> GETGQLIKDTIKNTVENTVESTHSISTEATPALQAAETGATSNASDESMIETRNVVNTHGVAETSLEGFYGRAGLVAMFTTEGGIRSWYINFGKYVQLRAKLELLTYARFDVEFTIVAQVVDEQAKVKDFNVDYQVMYVPPGASAPDGQ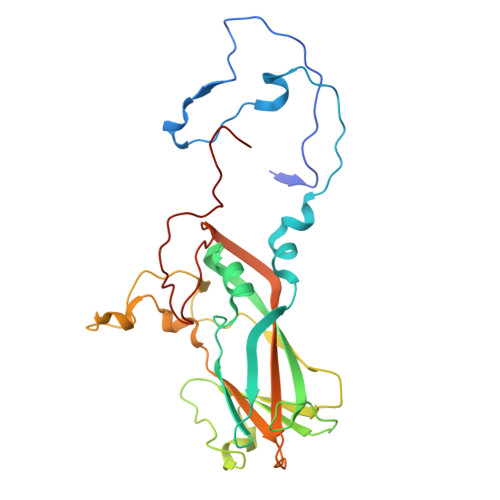DSFQWQSSCNPSVISNTGLPPARVSVPFMSSANAYSFSYDGYIQFGDTSSSSYGILPIHYLGQLVVRTCEDLDSARLRVRIYAKPKHMRGWIPRSPRMRPYVSRFTGIYTDAPSFCVNRESITTAG>MGLNIGDLLGSTPAKDQGCSRTCESQFCTIAPLLRYGKYCGILYSGCPGERPCDALDACCMVHDHCVDTHNDDYLN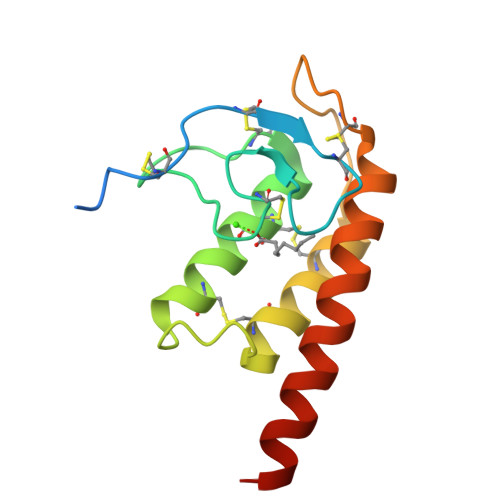TMCNENLLSCIDRVSGATFPGNKCNVGQTASVIRGVIETAVFAGKILHKRDDGQ[2x]> MITDWLPVWLLIALPAAGATILLLAGRRSDRWGHLLGCAMSLAAFAVGTVLFAGMLGRSGEERAVHEALFSWVPVGGLQVDFGLQLDQLSVCFVLLITGVGSLIHIYSIGYMAEDPDRRRFFAYLNLFLAAMLLLVLADNYLGLYAGWEGVGLASYLLIGFWSHKPSAATAAKKAFVVNRVGDMGLAIALMIMFATIGSISFAGVFAA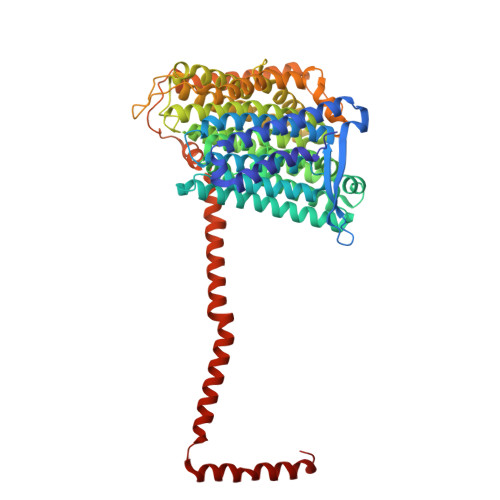APGLSEATLSAIGLLLLLGACGKSAQVPLQSWLGDAMEGPTPVSALIHAATMVTAGVYLIVRSGPIFDLAPTAQTGVVIVGAVTLLFGAIIGCAKDDIKKALAASTMSQIGYMVLAAGLGPAGYAFAIMHLLTHGFFKAGLFLGAGSVMHAMNDEVNMRRYGGLRKVLPVTFATFGLGYLAIIGVPPLAGFFSKDGIIEAALGAGGARGVILGGAAILGAGITAFYMTRVMLMTFFGEKRWAANSHPHEAPAVMTWPMILLAVGSVVSGGALAIGGTLSHWLEPVVGTHEAHHAVPVWVVTAIVLAVVAVGIAVAYRMYARQAVPEEVPEGSALTVAARRDLYGDAFNEAVFMRGGQTLTAAMVTVDDKAVDGTAGGLAALVSRTSDALRQVQTGFARSYALSMLGGSALVVAAILAVQLW Glycogen synthase (GYS1) is the central enzyme in muscle glycogen biosynthesis. GYS1 activity is inhibited by phosphorylation of its amino (N) and carboxyl (C) termini, which is relieved by allosteric activation of glucose-6-phosphate (Glc6P). We present cryo-EM structures at 3.0–4.0 Å resolution of phosphorylated human GYS1, in complex with a minimal interacting region of glycogenin, in the inhibited, activated and catalytically competent states. Each GYS1 monomer consisted of two Rossmann domains and a tetramerization domain and interacted with GYG1 in a 1:1 ratio.

We determined a 3.0 Å structure of a phosphorylated GYS1–GYG1ΔCD complex with D2 symmetry applied. The cryo-EM map ranged from 2.9 Å resolution at the core to 3.9 Å resolution at the periphery of the complex, allowing for modelling of residues 13–289, 293–629 and 637–645 of GYS1 and residues 317–349 of GYG1. The complex adopted a rectangular box shape, with residues 317–349 of GYG1 at each corner of the GYS1 homotetramer. In this structure, each GYS1 active site, at the cleft between the two Rossmann domains, was in a closed conformation owing to additional intersubunit contacts at a minor interface (B–D or A–C). The as-purified GYS1 was highly phosphorylated, representative of the T state and supported by the lack of GT activity without Glc6P. In the T state, the N and C termini from each subunit traversed from and toward the two regulatory α24 helices at the dimeric (C–D and A–B) interfaces, respectively. Although there was no clear density for phosphorylation sites 2 (Ser8) and 2a (Ser11), they would be positioned near the regulatory α24 helix of the subunit across the dimeric interface, close to both Arg579 and Arg580, which could potentially sense the phosphorylation at these sites. In both the C1 and D2 symmetry maps, strong density was apparent between Arg588 and Arg591 of both GYS1 subunits at the dimeric interface. We modelled a single phosphorylated site 3a (Ser641), which was the first C-terminal phosphorylation site in the sequence. Overall, our model suggests that the nonsymmetric interactions of a single phosphorylated site (3a) at the dimeric (C–D and A–B) interfaces, combined with intersubunit interactions of phosphorylated sites 2 and 2a across the interface, stabilize GYS1 in the inhibited state.

>[4x]MPLNRTLSMSSLPGLEDWEDEFDLENAVLFEVAWEVANKVGGIYTVLQTKAKVTGDEWGDNYFLVGPYTEQGVRTQVELLEAPTPALKRTLDSMNSKGCKVYFGRWLIEGGPLVVLLDVGASAWALERWKGELWDTCNIGVPWYDREANDAVLFGFLTTWFLGEFLAQSEEKPHVVAHFHEWLAGVGLCLCRARRLPVATIFTTHATLLGRYLCAGAVDFYNNLENFNVDKEAGERQIYHRYCMERAAAHCAHVFTTVSQITAIEAQHLLKRKPDIVTPNGLNVKKFSAMHEFQNLHAQSKARIQEFVRGHFYGHLDFNLDKTLYFFIAGRYEFSNKGADVFLEALARLNYLLRVNGSEQTVVAFFIMPARTNNFNVETLKGQAVRKQLWDTANTVKEKFGRKLYESLLVGSLPDMNKMLDKEDFTMMKRAIFATQRQSFPPVCTHNMLDDSSDPILTTIRRIGLFNSSADRVKVIFHPEFLSSTSPLLPVDYEEFVRGCHLGVFPSYYEPWGYTPAECTVMGIPSISTNLSGFGCFMEEHIADPSAYGIYILDRRFRSLDDSCSQLTSFLYSFCQQSRRQRIIQRNRTERLSDLLDWKYLGRYYMSARHMALSKAFPEHFTYEPNEADAAQGYRYPRPASVPPSPSLSRHSSPHQSEDEEDPRNGPLEEDGERYDEDEEAAKDRRNIRAPEWPRRASCTSSTSGSKRNSVDTATSSSLSTPSEPLSPTSSLGEERN;>MTDQAFVTLTTNDAYAKGALVLGSSLKQHRTTRRLVVLATPQVSDSMRKVLETVFDEVIMVDVLDSGDSAHLTLMKRPELGVTLTKLHCWSLTQYSKCVFMDADTLVLANIDDLFDREELSAAPDPGWPDCFNSGVFVYQPSVETYNQLLHLASEQGSFDGGDQGILNTFFSSWATTDIRKHLPFIYNLSSISIYSYLPAFKVFGASAKVVHFLGRVKPWNYTYDPKTKSVKSEAHDPNMTHPEFLILWWNIFTTNVLPLLQQFGLVKDTCSYVNVLSDLVYTLAFSCGFCRKEDVSGAISHLSLGEIPAMAQPFVSSEERKERWEQGQADYMGADSFDNIKRKLDTYLQ[4x]>DVYQEPTDPKFPQQWYLSGVTQRDLNVKAAWAQGYTGHGIVVSILDDGIEKNHPDLAGNYDPGASFDVNDQDPDPQPRYTQMNDNRHGTRCAGEVAAVANNGVCGVGVAYNARIGGVRMLDGEVTDAVEARSLGLNPNHIHIYSASWGPEDDGKTVDGPARLAEEAFFRGVSQGRGGLGSIFVWASGNGGREHDSCNCDGYTNSIYTLSISSATQFGNVPWYSEACSSTLATTYSSGNQNEKQIVTTDLRQKCTESHTGTSASAPLAAGIIALTLEANKNLTWRDMQHLVVQTSKPAHLNANDWATNGVGRKVSHSYGYGLLDAGAMVALAQNWTTVAPQRKCIIDILTEPKDIGKRLEVRKTVTACLGEPNHITRLEHAQARLTLSYNRRGDLAIHLVSPMGTRSTLLAARPHDYSADGFNDWAFMTTHSWDEDPSGEWVLEIENTSEANNYGTLTKFTLVLYGTASGSLVPRGSHHHHHH[4x];>GKRQFVNEWAAEIPGGPEAASAIAEELGYDLLGQIGSLENHYLFKHKNHPARSAASAFHITKRLSDDDRVIWAEQQYEKERSKR[4x]

Proprotein convertases (PCs), including furin and PC1/3 among nine mammalian homologues, mediate the maturation of numerous secreted substrates by proteolytic cleavage. The zymogens of the furin-like PCs share a multidomain architecture comprising an N-terminal pro-domain, a subtilisin-like catalytic domain, and a P-domain (also called HomoB-domain). Activation of furin is triggered by two sequential autocatalytic cleavages and subsequent release of the prodomain. In this work, we investigate the structural and functional basis of PC-activation to engineer prodomain-based PC-inhibitors.

The complementary triple mutant (77)A-R-S-A-A (M2) was also resistant to proteolysis by furin but revealed more potent inhibition compared to M1 (Ki = 0.32 ± 0.03 nM). Indeed, we could obtain crystals of M5:furin and M2:furin at pH 5.9 and pH 7.0, respectively. The structures of M2:furin and M5:furin were refined to 2.0 Å and 2.4 Å resolution, respectively. Four and three copies of the PC1/3-prodomain:furin complexes were observed in the asymmetric unit for M2:furin and M5:furin, respectively. In both complex structures, the globular part of the prodomain is bound to the western rim of the substrate binding pocket. The C-terminal residues 104-110 extend over all non-primed substrate binding pockets of furin (S1-S6). The main difference between M2:furin and M5:furin is found for the secondary cleavage site loop between Lys73 and Ala83. This region was well structured in M2:furin at pH 7.0, but no electron density was observed in M5:furin at pH 5.9. Apparently, the secondary cleavage site loop adopts a specific conformation at pH 7.0 but gets unstructured at pH 5.9. In the isolated structure of M2 and in the complex structure with furin, we found an unusual interaction of the His72 side chain with the amide nitrogen atoms of Asn74 and His75.>S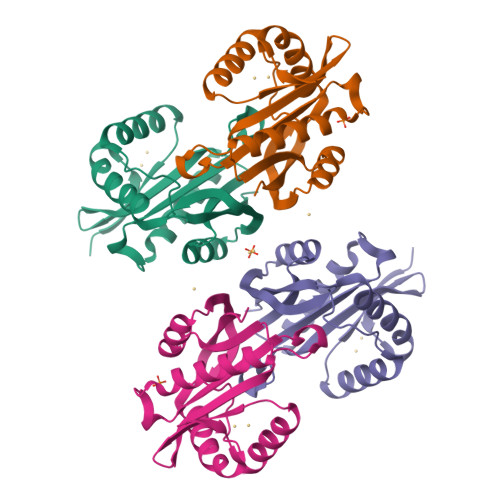NAMIRCAKKEDLNAILAIYNDAIINTTAVYTYKPQTIDERIAWFETKQRNHEPIFVFEENGSVLGFATFGSFRPWPAYQYTIEHSIYVDASARGKGIASQLLQRLIVEAKAKGYRTLVAGIDASNEASIKLHQKFNFKHAGTLTNVGYKFDYWLDLAFYELDLKD[2x]> XSGLDKYLPGIEKLRRGDGEVEVKSLAGKLVFFYFSASWCPPCRGFTPQLIEFYDKFHESKNFEVVFCTWDEEEDGFAGYFAKMPWLAVPFAQSEAVQKL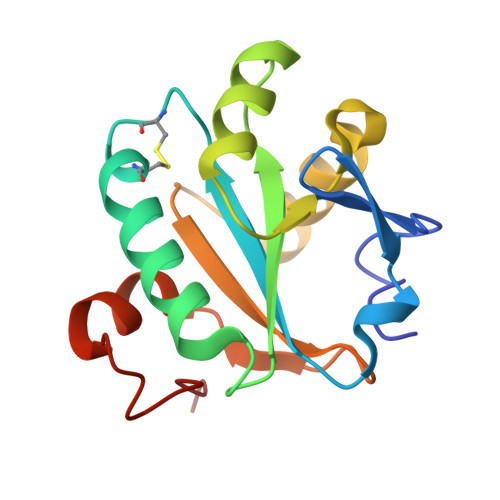SKHFNVESIPTLIGVDADSGDVVTTRARATLVKDPEGEQFPWKDAP>MGSSHHHHHHGSMQQLINSLFMEAFANPWLAEQEDQARLDLAQLVAEGDRLAFSTDSYVIDPLFFPGGNIGKLAICGTANDVAVSGAIPRYLSCGFILEEGLPMETLKAVVTSMAETARTAGIAIVTGDTKVVQRGAADKLFINTAGMGAIPTNIHWGAQTLTAGDILLVSGTLGDHGATILNLREQLGLDGELVSDCAVLTPLIQTLRDIPGVKALRDATRGGVNAVVHEFAAACGCGIEISESALPVKPAVRGVCELLGLDALNFANEGKLVIAVERNAAEQVLAALHSHPLGKDAALIGEVVERKGVRLAGLYGVKRTLDLPHAEPLPRI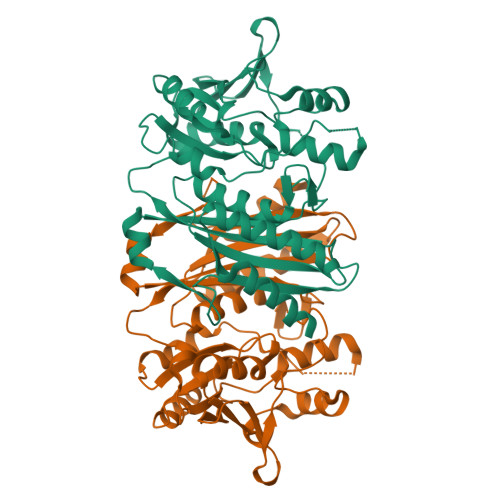C[4x]> MAGWNAYIDNLMADGTCQDAAIVGYKDSPSVWAAVPGKTFVNITPAEVGVLVGKDRSSFYVNGLTLGGQKCSVIRDSLLQDGEFSMDLRTKSTGGAPTFNVTVT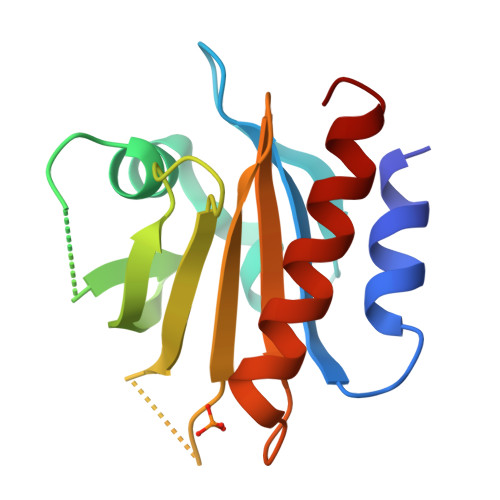KTDKTLVLLMGKEGVHGGLINKKCYEMASHLRRSQY4-{[(2S)-3,3-dimethyl-2-(pyridin-3-yl)-2,3-dihydro-1H-indol-1-yl]methyl}-N-hydroxybenzamide 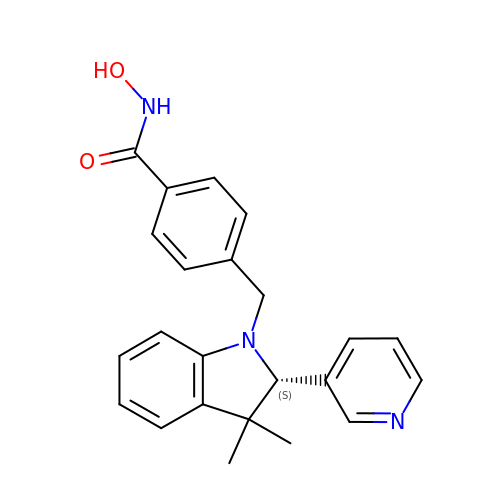| C23 H23 N3 O2 | HGCZGYHCBRKJNB-OAQYLSRUSA-N> MSQPQSSQVTKRGLTDPERAAIIAAAVPDHALDTQRKYHYFIQPRWKRLSEYEQLSCYAQPNPDWIAGGLDWGDWTQKFHGGRPSWGNESTELRTTDWYRHRDPARRWHHPYVKDKSEEARYTQRFLAAYSSEGSIRTIDPYWRDEILNKYFGALLYSEYGLFNAHSSVGRDCLSDTIRQTAVFAALDKVDNAQMIQMERLFIAKLVPGFDASTDVPK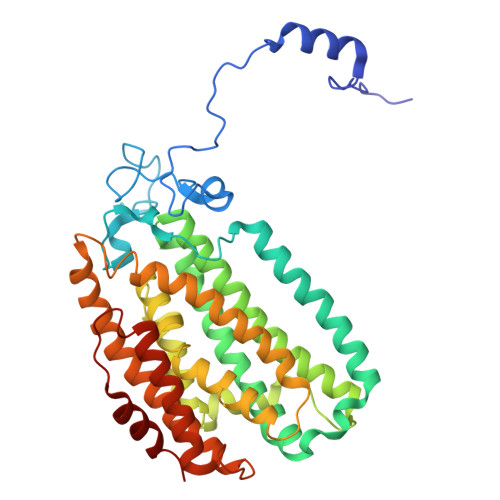KIWTTDPIYSGARATVQEIWQGVQDWNEILWAGHAVYDATFGQFARREFFQRLATVYGDTLTPFFTAQSQTYFQTTRGAIDDLFVYCLANDSEFGAHNRTFLNAWTEHYLASSVAALKDFVGLYAKVEKVAGATDRAGVSEALQRVFGDWKIDYADKIGFRVDVDQKVDAVLAGYKN Retaining α-glucosidases employ a conserved two-step Koshland double displacement mechanism, in which α-glucosidase substrates are hydrolyzed using two key carboxylic acid residues functioning as the catalytic nucleophile (Asp518 in GAA and Asp412 in CjAgd31B, a bacterial homologue of GAA) and catalytic acid/base (Asp616 in GAA and Asp480 in CjAgd31B). Mutations in the gene encoding for GAA can lead to enzyme deficiency which generates multiple phenotypic forms of the lysosomal storage disorder (LSD) Pompe disease (PD). Herein, we report a 1,6-epi-cyclophellitol cyclosulfamidate as a new class of reversible α-glucosidase inhibitors that displays enzyme inhibitory activity by virtue of its conformational mimicry of the substrate when bound in the Michaelis complex.

Crystallographic studies with the proteolytically digested form of human recombinant rhGAA (Myozyme)21 and the bacterial GH31 α-glucosidase/transglucosidase CjAgd31B homologue from Cellvibrio japonicus(30) further demonstrated the binding motifs of cyclosulfamidates 4 and 6. Similar assays with CjAgd31B using a Sypro Orange dye revealed that α-glc-cyclosulfamidate 4 stabilizes the bacterial analogue in vitro as well with a ΔTmmax of 5.2 °C and an EC50 of 134 μM. In conclusion, 1,6-epi-cyclophellitol cyclosulfamidate 4 is a selective reversible α-glucosidase ligand that binds through 4C1 conformational Michaelis complex mimicry.

> MNPVKREIHPDAVFYKEHKLRNDGLVITTNQGNIRLQFKSEAAIEVLYRADSKQLPSFALAQPESAIKAQLTETENHLQFSGGTLTARIQKRPFAISYYRDSELLLAEESGFQVNTDKINFRFYLSPGEKILGGGQRILGMDRRGQRFPLYNRAHYGYSDHSGQMYFGLPAIMSSKQYILVFDNSASGAMDIGKTESDILQLEAKSGRSAYILVAGNSYPSLIENFTQVTGRQPLPPRWALGSFASRFGYRSEAETRATVQKYKTEDFPLDTIVLDLYWFGKDIKGHMGNLDWDKENFPTPLDMMADFKQQGVKTVLITEPFVLTSSKRWDDAVKAKALAKDPQGQPKAFELYFGNGGIIDVFSKEGSRWFSSIYKDLSKQGVAGWWGDLGEPEMHPEDTQHAIGDADTVHNAYGHRWAEMLYQQQLDQFPELRPFIMMRAGFVGSQRYGMIPWTGDVSRTWGGLASQVELALQMSLLGFGYIHSDLGGFADGETLDKEMYIRWLQYGVFQPVYRPHGQDHIPSEPVFQDEETKAILRPLVKLRYRMLPYIYTAAYQNTLTGMPLMRPLFFSDEKNPALIDNKTSYFWGDSLLVTPITQAGVESVSIPAPKGVWFDFWKDTRYQTDGAPLTLPTDLHTIPVLVKAGAFMPYVPAVSTTEDYRSDSLEIHYYADASVPLAQGEIFEDDGKDPNSIKRNQFDLLTLQATHTDNQLHFQLARTGKGYRGMPERRATTLVIHNASDQYQHLDINGKTIAIAQADCASTPALACYDQERRQLQLVFTWGREALNLRLHKGGRADPAFLYKVVINSKLEGKPIPNPLLGLDSTRTGHHHHHH> AMPFEIEVLLPGEISPAETSALQKCEGKIITFSTLRHRASLVDIALSSYYING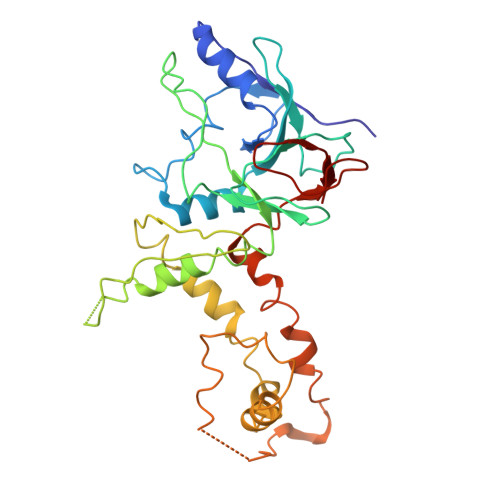APPDTLSLLEAYRMRFAAVITRVIPGKLLAHAIGVGTPTPGLFIQNTSPVDLCNGDYICLLPPVFGSADEIRLDSVGLEIVFPLTIPQTLMREIIAKVVARAVERTAAGRTPGELPGADVICYNGRRYELETNLQHRDGSDAAIRTLVLNLMFSINEGTTLILTLITRLLVQGAHDGYVNLLIQTANCVRETGQPMPRIQDGHRRFPIYEAISSWISTSSRLGDTLGTRAILRVCVFDGPSTVHPGDRTAVIQV>M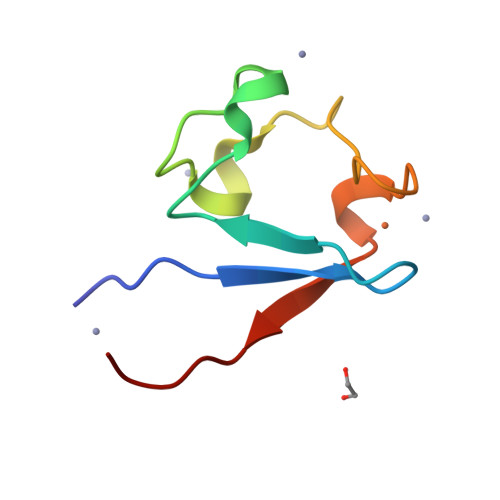NDYKLFRCIQCGFEYDEALGWPEDGIAAGTRWDDIPDDWSCPDCGAAKSDFEMVEVARS[8x]(2~{S})-4-[[(2~{R},3~{S},4~{R},5~{R})-5-(6-aminopurin-9-yl)-3,4-bis(oxidanyl)oxolan-2-yl]methyl-[2-[[9-[(2~{R},3~{R},4~{S},5~{R})-5-(hydroxymethyl)-3,4-bis(oxidanyl)oxolan-2-yl]purin-6-yl]amino]ethyl]amino]-2-azanyl-butanoic acid | C26 H36 N12 O9 | 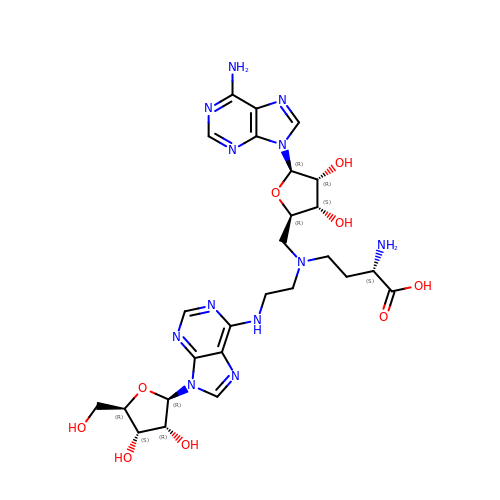UAGVZMOWWSWEAM-CZUOOHDMSA-N>MTHHYPTDDIKIKEVKELLPPIAHLYELPISKEASGLVHRTRQEISDLVHGRDKRLLVIIGPCSIHDPKAALEYAERLLKLRKQYENELLIVMRVYFEKPRTTVGWKGLINDPHLDGTFDINFGLRQARSLLLSLNNMGMPASTEFLDMITPQYYADLISWGAIGARTTESQVHRELASGLSCPVGFKNGTDGNLKIAIDAIGAASHSHHFLSVTKAGHSAIVHTGGNPDCHVILRGGKEPNYDAEHVSEAAEQLRAAGVTDKLMIDCSHANSRKDYTRQMEVAQDIAAQLEQDGGNIMGVMVESHLVEGRQDK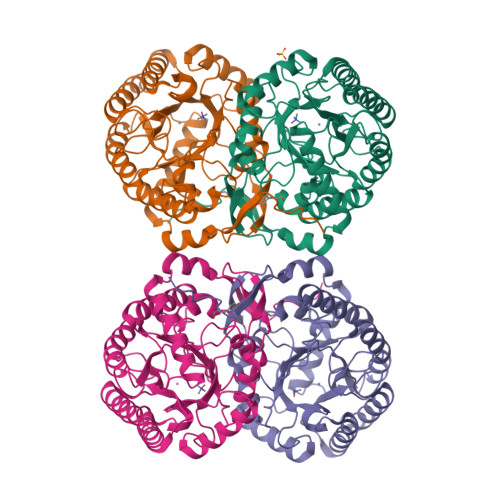PEVYGKSITDACIGWGATEELLALLAGANKKRMARAS[4x]BusR is a member of a yet structurally uncharacterized subfamily of the GntR family of transcription factors that downregulates transcription of the genes for the BusA (OpuA) glycine-betaine transporter upon c-di-AMP binding. BusR satisfies the overall domain architecture of the GntR family with its N-terminal winged helix-turn-helix motif (wHTH) and a C-terminal effector binding motif, an RCK_C domain (regulator of K+ conductance). Our structural data, supported by biochemical and biophysical data, reveal that BusR utilizes a unique domain assembly with a tetrameric coiled-coil in between the binding platforms, serving as a molecular ruler to specifically recognize a 22 bp separated bipartite binding motif. Binding of c-di-AMP to BusR induces a shift in equilibrium from an inactivated towards an activated state that allows BusR to bind the target DNA, leading to transcriptional repression.

Thus, to visualize this ternary complex of c-di-AMP activated BusR on dsDNA, we solved two complex structures by single-particle cryo-electron microscopy. One structure contains BusR bound to pAB1 at a resolution of 7.1 Å and the other structure was determined using the whole promotor sequence (pAB, two BusR binding sites). While the resolution of the EM density is not good enough to determine the register of the DNA directly, it can be deduced from the lower resolution BusR:c-di-AMP:pAB1 structure, as the whole dsDNA density (46 bp) is visible. As expected, BusR binds to the DNA as a tetramer, which reflects the oligomeric assembly we observed by SEC-RALS and SAXS in solution. Compared to the crystal structure, BusR undergoes major structural rearrangements upon binding to dsDNA. The central coiled-coils align in an ‘X’-like fashion relative to the dsDNA. In our structure, BusR induces a bending of the DNA by ∼18°. The Helices αG2 and αG3 of wHTHinhib plunge deep into the major groove, in close contact to the motif sequence, while the ‘wing’ of wHTHinhib (loop between βG1 and βG2) reaches into the minor groove. In this complex, wHTHfree faces the DNA in the same orientation as wHTHinhib but is positioned one quarter of a DNA turn (90°) further inwards, towards the middle of the DNA sequence. Based on our structure, wHTHfree appears to be limited to phosphate backbone contacts.

>GPMVSEQSEIVTSKYQKIAVAVAQRIANGDYEVGEKLKSRTTIASTFNVSPETARKGLNILADLQILTLKHGSGAIILSKEKAIEFLNQYETSHSVAILKGKIRDNIKAQQQEMEELATLVDDFLLQTRAVSKQYPLAPYEIIVSEDSEHLGKSIGELNVWHQTGATIVAIEHEGKFIVSPGPFSVIEQGDHIFFVGDEDVYARMKTYFNLRMGL[4x]methyl N-[(2S)-2-({(S)-hydroxy[(1R)-3-methyl-1-{[N-(3-methylbutanoyl)-L-valyl-L-valyl]amino}butyl]phosphoryl}oxy)-3-phenylpropanoyl]-L-alanyl-L-alaninate 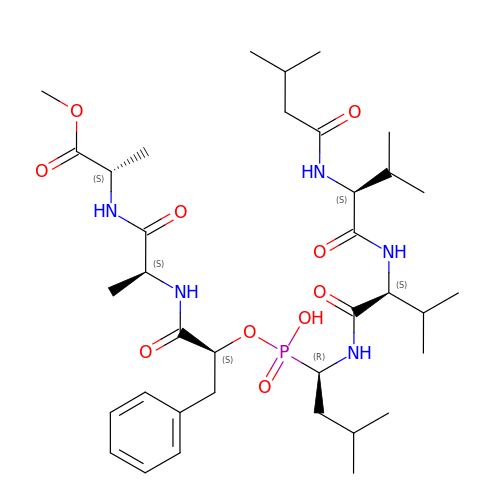| C36 H60 N5 O10 P | CEPZPGMVMASQKU-ORDNGIEBSA-N>[2x]SRAPYSGPQDLAALLEQIGCLKY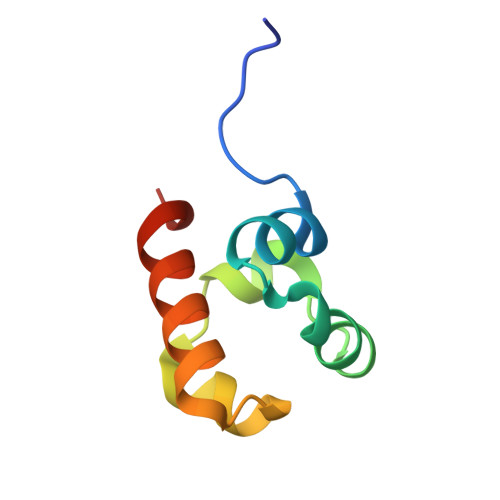LQVFEEQDVDLRIFLTLTESDLKEIGITAFGPKRKMTSAIARWHSSAR ISOBUTYRYL-COENZYME A | C25 H42 N7 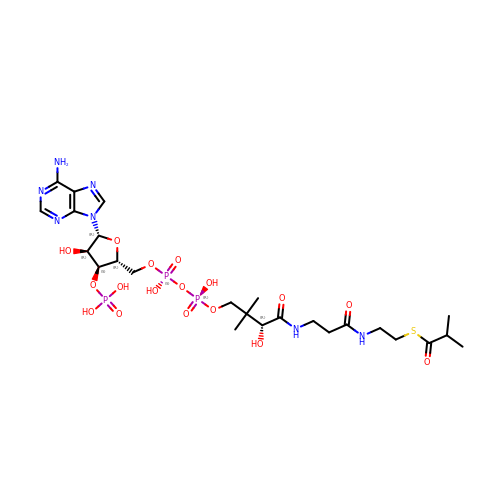O17 P3 S | AEWHYWSPVRZHCT-NDZSKPAWSA-N>[2x]MRMTWNFHQYYTNRNDGLMGKLVLTDEEKNNLKALRKIIRLRTRDVFEEAKGIAKAVKKSALTFEIIQEKVSTTQIKHLSDSEQREVAKLIYEMDDDARDEFLGLTPRFWTQGSFQYDTLNRPFQPGQEMDIDDGTYMPMPIFESEPKIGHSLLILLVDASLKSLVAENHGWKFEAKQTCGRIK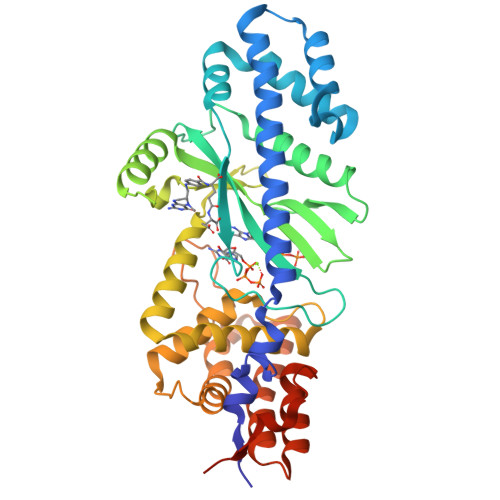IEAEKTHIDVPMYAIPKDEFQKKQIALEANRSFVKGAIFESYVADSITDDSETYELDSENVNLALREGDRKWINSDPKIVEDWFNDSCIRIGKHLRKVCRFMKAWRDAQWDVGGPSSISLMAATVNILDSVAHDASDLGETMKIIAKHLPSEFARGVESPDSTDEKPLFPPSYKHGPREMDIMSKLERLPEILSSAESADSKSEALKKINMAFGNRVTNSELIVLAKALPAFAQELEHHHHHH>AIILGIDPGSRVTGYGVIRQVGRQLSYLGSGCIRTKVDDLPSRLKLIYAGVTEI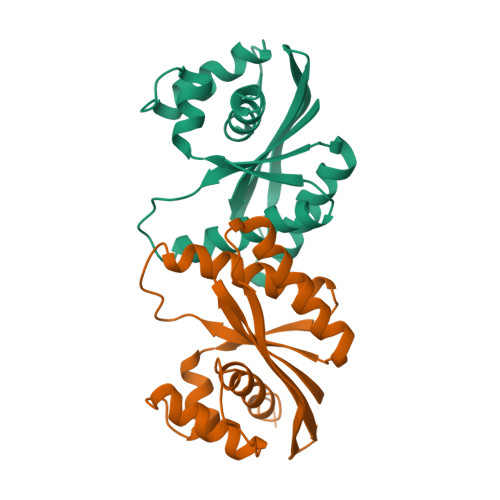ITQFQPDYFAIEQVFMAKNADSALKLGQARGVAIVAAVNQELPVFEYAARQVKQTVVGIGSAEKSQVQHMVRTLLKLPANPQADAADALAIAITHCHVSQNAMQ[4x]>[2x]AVEQCDLSQFQTTSSNQLMAAIRQQGASCVNALFSADTGVQEAAFSSNHMYNVAQYTRTLAQQYAGGGSDELEALYLYLRAGYYAEFYNSNITFLSWVTPAVKGAVDAFVQNAHFYDNGDAHGKVLNEVIITMDSAGLQHAYLDVVTQWLTRWNAQYAEHWYMRNAVNGVFTLLFGGQWNNQYTSLIGEQTALVTALQAFALDRTKVNSPTEFMAANAARELGRLARYTDATIAPKVTEGLTAIFGQYPSYGDGDAIWLGAADTASYYADCSQFNICGFEDALRDAALNQTFICSDTIKIRSQDM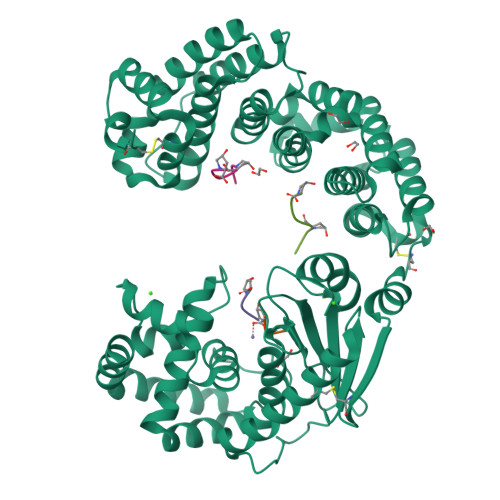SQAQHLAACDKMAYEESFFHTTLETGNQPVADDHNTQLQVNIFNSDTDYGKYAGPIFGIDTNNGGMYLEGNPANVGNIPNFIAYEASYANPDHFVWNLEHEYVHYLDGRFNMYGDFGTPTELVVWWSEGVAEYVSRVNDNPQAIATIQDGSTYTLAQVFDTTYDGFDVDRIYRWGYLAVRFMFERHPDEVQRMLSATRQGRWAEYKAIISGWANQYQSEFAQWTEALAKGDSGAGNGEGTGSGNEGGGESGGNT;>[4x]GPP;>[4x]GPPGPP> ALPAWARPDYNPPLVE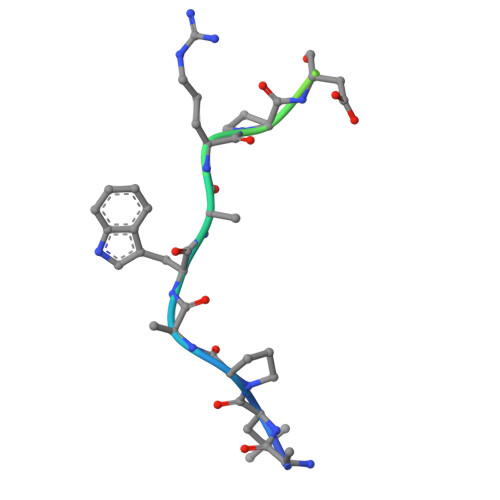SWRR>[4x]XLAAA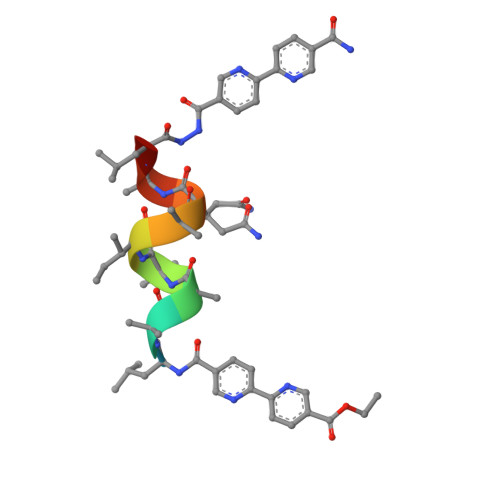IAQALX>[2x]GAMSTLGDLLAEHTVLPGSAVDHLHAVVGEWQLLADLSFADYLMWVRRDDGVLVCVAQCRPNTGPTVVHTDAVGTVVAANSMPLVAATFSGGVPGREGAVGQQNSCQHDGHSVEVSPVRFGDQVVAVLTRHQPELAARRRSGHLETAYRLCATDLLRMLAEGTFPDAGDVAMSRSSPRAGDGFIRLDVDGVVSYASPNALSAYHRMGLTTELEGVNLIDATRPLISDPFEAHEV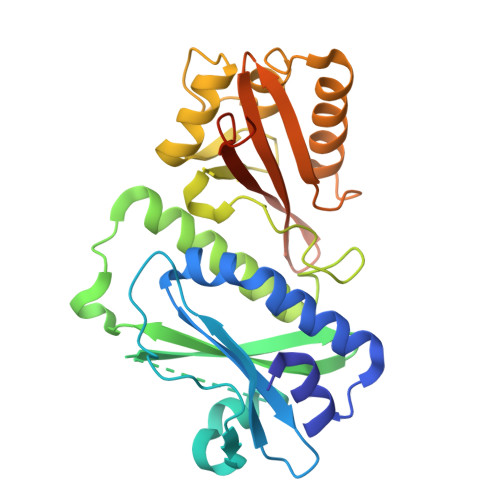DEHVQDLLAGDGKGMRMEVDAGGATVLLRTLPLVVAGRNVGAAILIRDVTEVKRRDRALISKDATIREIHH> GPPGEVMGRAIARVADTIGSGPVNSESIPALTAAETGHTSQVVPSDTMQTRHVKNYHSRSESTVENFLCRSACVFYTTYENHDSDGDNFAYWVINTRQVAQLRRKLEMFTYARFDLELTFVITSTQEQPTVRGQDAPVLTHQIMYVPPGGP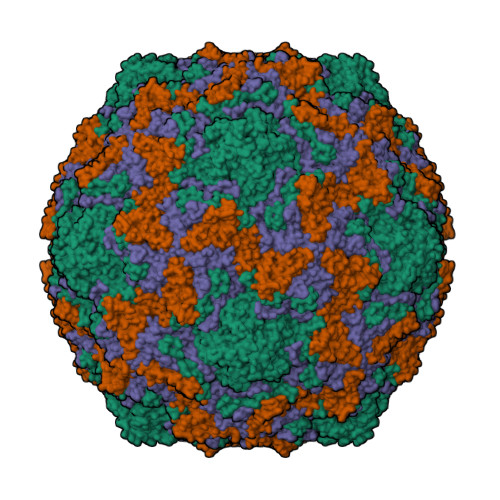VPTKVNSYSWQTSTNPSVFWTEGSAPPRMSVPFIGIGNAYSMFYDGWARFDKQGTYGISTLNNMGTLYMRHVNDGGPGPIVSTVRIYFKPKHVKTWVPRPPRLCQYQKAGNVNFEPTGVTEGRTDITTMKTT;> SPSAEECGYSDRVRSITLGNSTITTQECANVVVGYGVWPTYLKDEEATAEDQPTQPDVATCRFYTLESVMWQQSSPGWWWKFPDALSNMGLFGQNMQYHYLGRAGYTIHVQCNASKFHQGCLLVVCVPEAEMGCATLANKPDPKSLSKGEIANMFESQNSTGETAVQANVINAGMGVGVGNLTIFPHQWINLRTNNSATIVMPYINSVPMDNMFRHNNFTLMVIPFAPLSYSTGATTYVPITVTVAPMCAEYNGLRLAGKQ;> GLPTLSTPGSNQFLTSDDFQSPSAMPQFDVTPEMDIPGQVNNLMEIAEVDSVVPVNNTEGKVMSIEAYQIPVQSNPTNGSQVFGFPLTPGANSVLNRTLLGEILNYYAHWSGSIKLTFMFCGSAMATGKFLLAYSPPGAGAPTTRKEAMLGTHVIWDVGLQSSCVLCIPWISQTHYRYVVMDEYTAGGYITCWYQTNIVVPADAQSDCKILCFVSACNDFSVRMLKDTPFIKQDNFFQ;> MGAQVSTQKTGAHETSLSAAGNSVIHYTNINYYKDAASNSANRQDFTQDPGKFTEPVKDIMVKSMPALN To generalize this engineering approach for crystal contacts, a non-ADH-homologous enzyme was selected to apply the established strategies to the Nostoc sp. PCC 1720 ene reductase (NostocER). This oxidoreductase from the old yellow enzyme family (OYE, EC 1.6.99.1) catalyzes the trans-hydrogenations of activated alkenes, demonstrating its industrial relevance as a biocatalyst. As OYEs are strongly dependent on cost-intensive NADPH as a cofactor, Mähler et al. engineered NADH-accepting variants (NostocER1) by exchanging NostocER loop regions at cofactor-binding sites to ER loop regions from Achromobacter sp. JA81 and Acaryochloris marina with a higher NADH affinity. For this study, the NostocER1 Loop1,5 variant (NostocER1-L1,5) was selected as an example protein for the rational introduction of Lys–Glu interactions at crystal contacts to demonstrate the impact of rational single amino acid exchanges on the crystallizability of proteins and enhance protein crystallization.

Out of the crystallization conditions resulting in crystals within two days, the following were selected based on cost efficiency and compatibility for customers and the environment: 25 mM Tris–HCl, 0.1 M NH4Cl, 5 mM CaCl2·2H2O, 50–150 g L−1 PEG 6000, pH 8.5. X-ray diffraction analysis performed on crystals taken from µL-batch experiments revealed a crystal structure with a resolution of 1.27 Å (see Section 2.5). Based on the observed intermolecular crystal contacts, nine amino acids were selected for NspER1-L1,5 mutation. They were selected based on their distance to a potential intermolecular interaction partner at the crystal contact of <6 Å (except for Q263K). Exemplarily, the NspER1-L1,5 crystal contact at positions 204 and 350–353 is depicted below, with mutations Q204K and Q350K/D352K/T354K generated in silico and the distance between the potential interacting amino acid residues E89 and E25/27, respectively, calculated using PyMOL (v.2.3). However, for the NspER1-L1,5 WT, no crystals were visible with the Tris buffer, and a lower number of larger crystals (compared to mutant Q204K) grew with the HEPES buffer. Contrary to the Q204K mutant, the addition of PEG 6000 did not initiate the NspER1-L1,5 WT crystallization in a stirred 5 mL crystallizer. Its concentration in the liquid phase remained nearly constant throughout the process. In accordance with the protein concentration measurements, no crystals were observed in the crystallization samples of the NspER1-L1,5 WT after 20.5 h of crystallization.

>[2x]MGHHHHHHGSGSTNINLFSSYQLGELELPNRIVMAPLTRSRAGEGNVPHQLNAIYYGQRASAGLIIAEATQVTPQGQGYPHTPGIHSPEQVAGWKLVTDTVHQQGGRIFLQLWHVGRISHPDLQPDGGLPVAPSAIAPKGEVLTYEGKKPYVTPRALDTSEIPAIVEQYRQGAANALAAGFDGVEIHAANGYLIDQFLRDGTNQRTDEYGGAIENRARLLLEVTEAITSVWDSQRVGVRLSPLTTLNGCVDSHPLETFGYVAQALNRFNLSYLHIFEAIDADIRHGGTVVPTSHLRDRFTGTLIVNGGYTREKGDTVIANKAADLVAFGTLFISNPDLPERLEVNAPLNQADPTTFYGGGEKGYTDYPFLAVANK> SNAMSKRVLMVVTNHTTITDDHKTGLWLEEFAVPYLVFQEKGYDVKVASIQGGEVPLDPRSINEKDPSWAE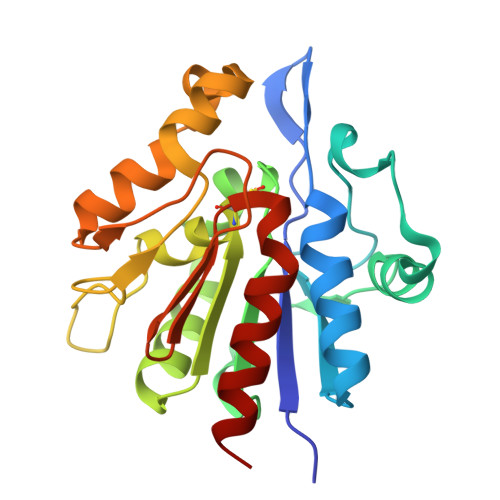AEAALKHTARLSKDDAHGFDAIFLPGGHGTMFDFPDNETLQYVLQQFAEDGRIIAAVCHGPSGLVNATYKDGTPIVKGKTVTSFTDEEEREVGLDVHMPFLLESTLRLRGANFVRGGKWTDFSVRDGNLITGQNPQSSRSTAEKVVAALEERE In particular, l-lysine decarboxylase (LDC) is an important enzyme for the biosynthesis of cadaverine, which is a crucial platform chemical with many industrial applications. In this report, we determined the crystal structures of LDC from Selenomonas ruminantium (SrLDC) in different crystallization conditions and observed that high flexibility of the PLP binding site seems to be one of the factors that lead to the low affinity for PLP in SrLDC. The monomeric form of SrLDC consists of two distinct domains, a PLP-binding barrel domain, and a sheet domain. The SrLDC homodimer is formed by a head-to-tail contact between the barrel domain of one monomer and the sheet domain of the other monomer.

To reveal the molecular mechanism of SrLDC, we determined its crystal structure at 2.0 Å resolution. The asymmetric unit contains one SrLDC molecule, and the dimeric structure of the protein could be easily generated by applying crystallographic P43212 symmetry. When we superimpose the structure of the apo-form of SrLDC in P43212 space group with that of SrLDC complexed with PLP/cadaverine, the overall shape of the two structures is almost the same, with an R.M.S.D. value of 0.72 Å. However, remarkable structural differences are observed at the active site. Interestingly, in the structure of the apo-form of SrLDC, the connecting loop between β-7 and α-8 (Phe178-Thr187) moved away from the PLP binding site by a distance of 5.0 Å, compared with the structure of SrLDC complexed with PLP/cadaverine. Because the conformational change disrupts these hydrogen bonds between the loop and the phosphate moiety of PLP, it might severely impair binding of the cofactor to the protein. Also interestingly, the conformational change of the PS-loop subsequently causes a more dramatic conformational change in the loop connecting β-8 and α-9 (Phe220-Asp231). The loop, located near the PLP binding site in the structure of SrLDC complexed with PLP/cadaverine, moved away from the PLP binding site by a distance of 12.2 Å in the structure of the apo-form. In contrast, in the apo-form of SrLDC, the loop is stabilized by the N-terminal region instead: the main-chains of Met1 and Leu228 form a hydrogen bond with each other, and the main-chains of Pro223 and Ala225 form hydrogen bonds with both the side- and the main-chains of Asn3.

> MKNFRLSEKEVKTLAKRIPTPFLVASLDKVEENYQFMRRHLPRAGVFYAMKANPTPEILSLLAGLGSHFDVASAGEMEILHELGVDGSQMIYANPVKDARGLKAAADYNVRRFTFDDPSEIDKMAKAVPGADVLVRIAVRNNKALVDLNTKFGAPVEEALDLLKAAQDAGLHAMGICFHVGSQSLSTAAYEEALLVARRLFDEAEEMGMHLTDLDIGGGFPVPDAKGLNVDLAAMMEAINKQIDRLFPDTAVWTEPGRYMCGTAVNLVTSVIGTKTRGEQPWYILDEGIYGCFSGIMYDHWTYPLHCFGKGNKKPSTFGGPSCDGIDVLYRDFMAPELKIGDKVLVTEMGSYTSVSATRFNGFYLAPTIIFEDQPEYAARLTEDDDVKKKAAV>[6x]MTVTLKQHERPAASRIVAVGAYRPANLVPNEDLIGPIDSSDEWIRQRTGIVTRQR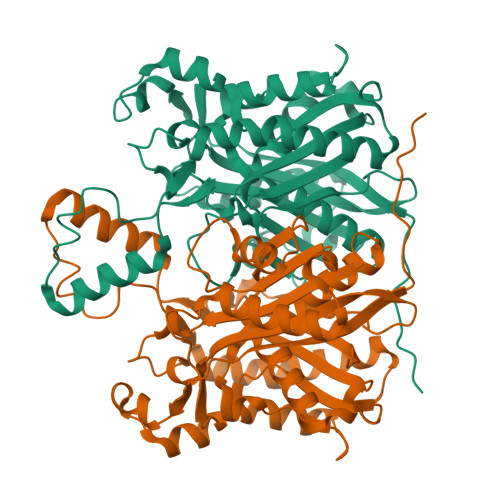ATAEETVPVMAVGAAREALERAGLQGSDLDAVIVSTVTFPHATPSAAALVAHEIGATPAPAYDVSAACAGYCYGVAQADALVRSGTARHVLVVGVERLSDVVDPTDRSISFLLGDGAGAVIVAASDEPGISPSVWGSDGERWSTISMTHSQLELRDAVEHARTTGDASAITGAEGMLWPTLRQDGPSVFRWAVWSMAKVAREALDAAGVEPEDLAAFIPHQANMRIIDEFAKQLKLPESVVVARDIADAGNTSAASIPLAMHRLLEENPELSGGLALQIGFGAGLVYGAQVVRLP> MLIRAFIPAHITAFFVPVFHEEPLKAGSLGAGVNLSKGTNVFASIETGTLERHIHVAFNGEPVKREEAEITYYVAEKLVPKDFLGEVEVWQYFDFPNGYGFGNSAGGALGTALALSYAFGGTWLRAAQLAHEAEVKHKGGLGDVIGQLAGGIEVRIKPGGPGIGVTDNLFFEDYKVLVVPLGRLSTREVLDGDVVKAIEVEGRKALEELLKEPKPERMMVLARNFAEKTGLLPGELSEIARELDKVLKNPSSMIMLGKGLFALVRDEEAEKAKQLLSDMNLPYD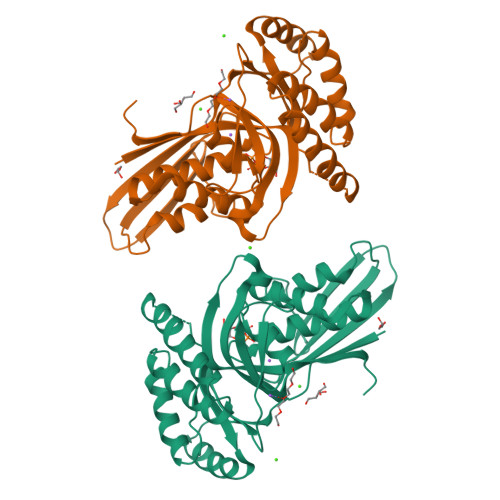IAEIYTERPKVGRWVG> MTTSDLVAGELAGDGLRDTRPGDTWLADRSWNRPGWTVAELEAAKAGRTISVVLPALDEEDTIGSVIDSISPLVDGLVDELIVLDSGSTDDTEIRAVAAGARVVSREQALPEVPIRPGKGEALWRSLAASRGDIVVFVDSDLINPHPMFVPWLVGPLLTGDGVHLVKSFYRRPLNVGDAGGGAGATGGGRVTELVARPLLAALRPE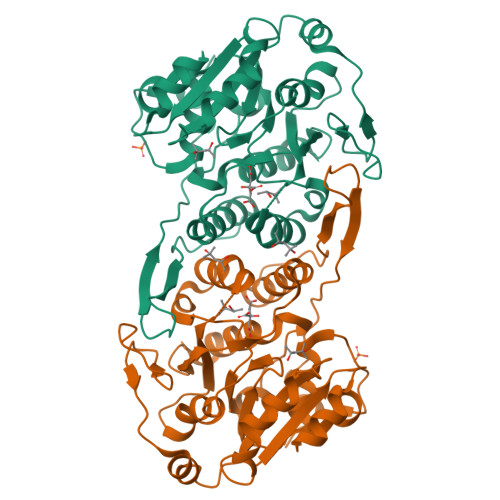LGCILQPLGGEYAATRELLTSVPFAPGYGVEIGLLVDTFDRLGLDAIAQVNLGVREHRNRPLAELGAMSRQVIATLLSRCGIPDSGVGLTQFVADGPEGQSYTQHTWPVSLADRPPMQAIRPR> MRLFVSDGVPGCLPVLAAAGRARGRAEVLISTVGPQDCVVPFLTRPKVPVLQLDSGNYLFSTSAICRYFFLLSGWEQDDLTNQWLEWEATELQPALSAALYYLVVQGKKGEDVLGSVRRALTHIDHSLSRQNCPFLAGETESLADIVLWGALYPLLQDPAYLPEELSALHSWFQTLSTQEPCQRAAQTVLKQQGVLALRPYLQKQPQPSPAEGRAVTNEPEEEELE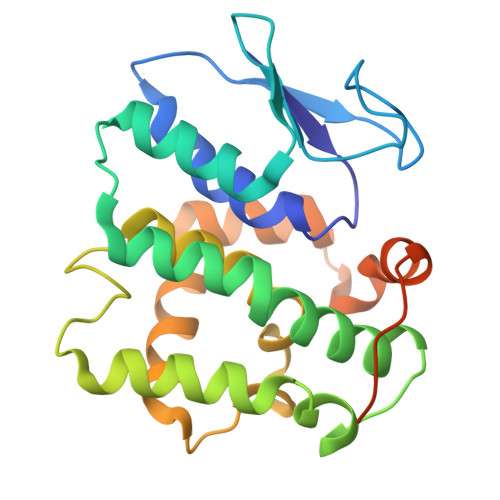HHHHHH>GAMDPEAAALRAELRDLELEEARLVQELEDVDRNNARAAADLQAAQAEAAELDQQERQHYRDYSALKRQQLELLDQLGNVENQLQYARVQRDRLK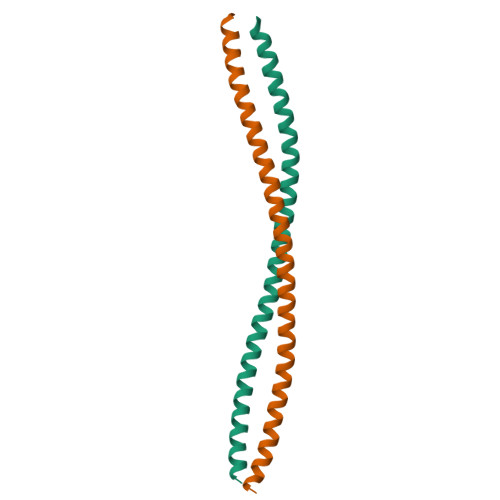EIN[4x]> CT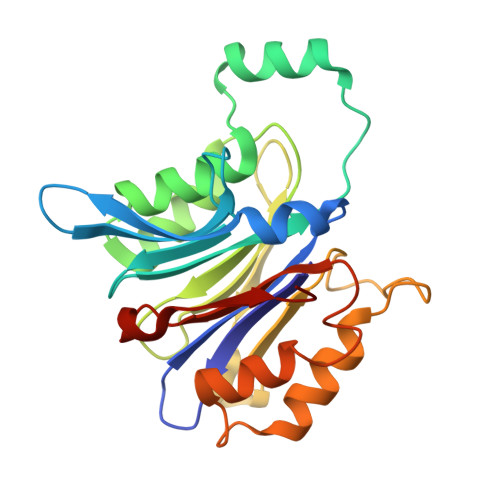SVVAQDSRGHIYHGRNLDYPFGDLLRKMTVDVQFLKNGQIAFTGTTFIGYVGLWTGQSPYKFTVSGDERADKGWWWENMIAALFQGHSPVSWLIRTTLSESEDFEASVYKLAKTPLIADVYYIVGGTAPGEGVVVTRNRGGPADIWPLDPLNGAWFRVETNYDHWKPVPKSDDRRTPAIKALNATGQANLSLEALFQVLSVVPVCNKITVYTTVMSAATPDKYMTRIRNLS> ADSTITIRGYVRDNGCSVAAESTNFTVDLMENAAKQFNNIGATTPVVPFRILLSPCGNAVSAVKVGFTGVADSHNANLLALENTVSAASGLGIQLLNEQQNQIPLNAPSSALSWTTLTPGKPNTLNFYARLM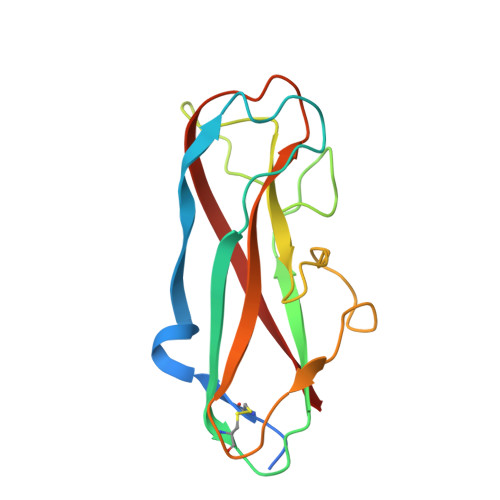ATQVPVTAGHINATATFTLEYQ> MAEVLSLVDLEIPQVTDKYYKFDTFKHLICHLFKKTSTETDSNVPIVIIFPTNNDIPSRKTRSTTTTTTTTTTTNTSKLDNLPFSDKSLLIQFFFTHLNILMIQGENSDEGKLYQEISSAKELLTNRISRVGNWTGTTHFRYCRHENDCGLLNQHSKIAGIIPTMTYILNCNATRSEIATNQLIYLYRLMIEEINFIELLQDASTTRLSQLCYAVGHWSFPAHNLSNDDLVYCVYLMIDYAIKQVEGFDNIPLNELLAFIFIVRDTYKNGNPFHNFRHAVDVLQACFHFLIRLGSLPKFKQFVEDPKLDYTEVHDKHTVLIALQNNSSEEKASLNPIQTLGLLVAALGHDVGHPGTTNDFMIKFSAPTALLYNDRSVLESYHASLFINKVLR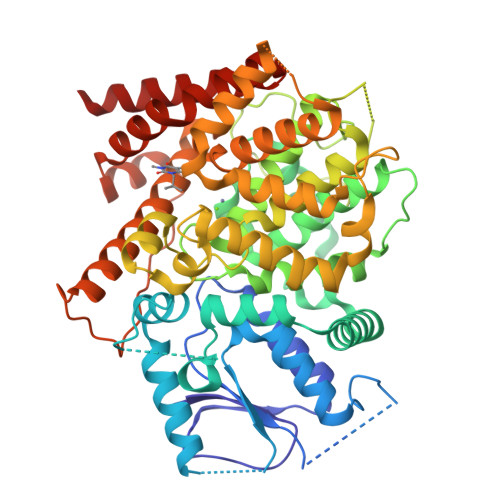ICWPDLLTCTIEEKSELTIRSLIISSILATDMGEHNEYVNRLKSFKTHNEILNHDNTVKLISALLIKCADISNVTRPLRVSAQWAMVLSREFAEVELLKSVIKKDIDLDFTKDLTYDDVPHELREILEIQPDIHKGQIFFINLFAENLFNSVSDLLPQLQYTCDIIMENKLFWLERAKK>[2x]MIEPFGNQYIVARPVYSTNAFEENHKKTGRHHKTFLDHLKVCCSCSPQKAKRIVLSLFPIASWLPAYRLKEWLLSDIVSGISTGIVAVLQGLAFALLVDIPPVYGLYASFFPAIIYLFFGTSRHISVGPFPILSMMVGLAVSGAVSKAVPDRNATTLGLPNNSNNSSLLDDERVRVAAAASVTVLSGIIQLAFGILRIGFVVIYLSESLISGFTTAAAVHVLVSQLKFIFQLTVPSHTDPVSIFKVLYSVFSQIEKTNIADLVTALIVLLVVSIVKEINQRFKDKLPVPIPIEFIMTVIAAGVSYGCDFKNRFKVAVVGDMNPGFQPPITPDVETFQNTVGDCFGIAMVAFAVAFSVASVYSLKYDYPLDGNQELIALGLGNIVCGVFRGFAGSTALSRSAVQESTGGKTQIAGLIGAIIVLIVVLAIGFLLAPLQKSVLAALALGNLKGMLMQFAEIGRL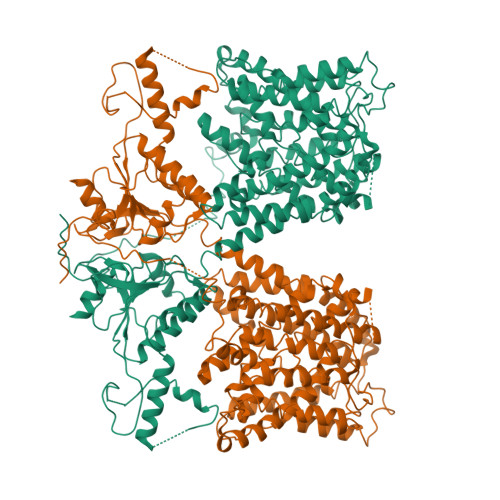WRKDKYDCLIWIMTFIFTIVLGLGLGLAASVAFQLLTIVFRTQFPKCSTLANIGRTNIYKNKKDYYDMYEPEGVKIFRCPSPIYFANIGFFRRKLIDAVGFSPLRILRKRNKALRKIRKLQKQGLLQVTPKGFICTVDTIKDSDEELDNNQIEVLDQPINTTDLPFHIDWNDDLPLNIEVPKISLHSLILDFSAVSFLDVSSVRGLKSILQEFIRIKVDVYIVGTDDDFIEKLNRYEFFDGEVKSSIFFLTIHDAVLHILMKKDYSTSKFNPSQEKDGKIDFTINTNGGLRNRVYEVPVETKF> GSVHKHTGRNCGRKFKIGEPLYRCHECGCDDTCVLCIHCFNPKDH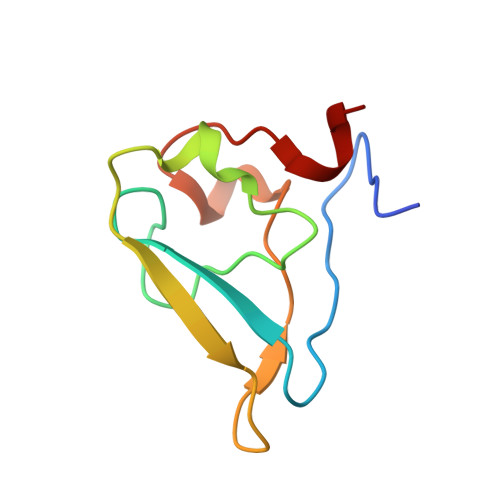VNHHVCTDICTEFTSGICDCGDEEAWNSPLHCKAEEQ>[2x]HHENLDISPSEVNGDWRTLYIVADNVEKVAEGGSLRAYFQHMECGDECQELKIIFNVKLDSECQTHTVVGQKHEDGRYTTDYSGRNYFHVLKKTDDIIFFHNVNVDESGKET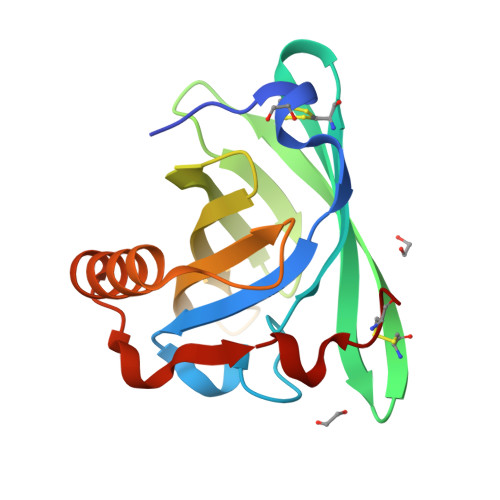NVILVAGKREDLNKAQKQELRKLAEEYNIPNENTQHLVPTDTCNQ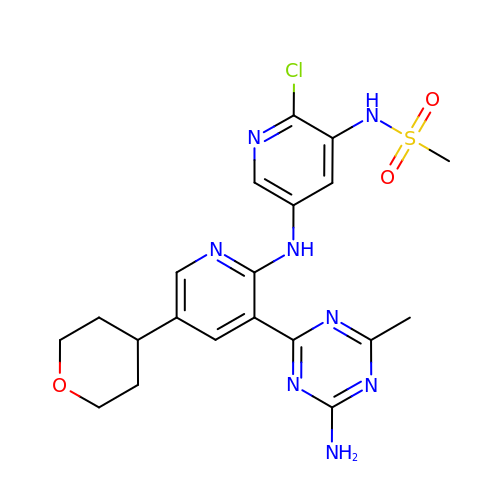N-(5-{[3-(4-amino-6-methyl-1,3,5-triazin-2-yl)-5-(tetrahydro-2H-pyran-4-yl)pyridin-2-yl]amino}-2-chloropyridin-3-yl)methanesulfonamide | C20 H23 Cl N8 O3 S | FLBPZSHGOYHCPK-UHFFFAOYSA-N>MGSSHHHHHHSQDPMSLLARLAPHLPYIRRYARALTGDQATGDHYVRVALEALAAGELVLDANLSPRVALYRVFHAIWLSSAGDDAAQRLMRIAPRSRQAFLLTALEGFTPTEAAQILDCDFGEVERLIGDAQAEIDAELAT[2x];>[2x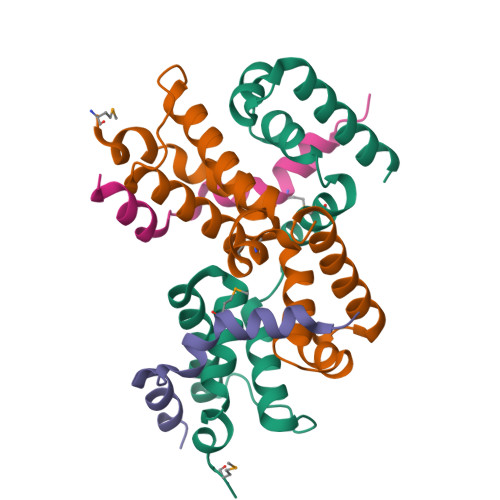]MNFGVEDMIEHVPMEDKRKGAAALDEARLRQQAIGVKLRQMFDEVVNEPVPDEFLAILRKAERPAGGE> GE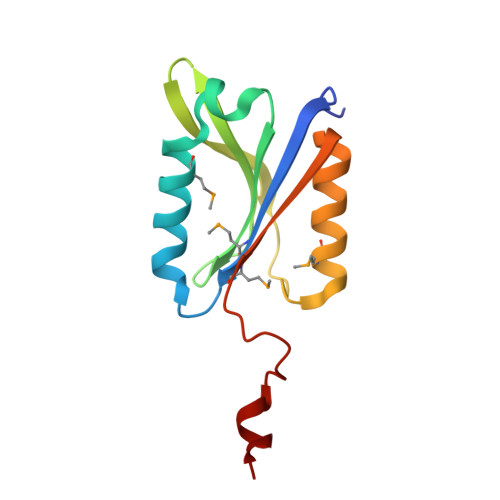TPEPRTTRTILVYMMANNSLNSFASKNIESMIEGATSKNLNGGNLIVYYAPAGSPPELLRIKEENGVVKKIHLKDYEKQNSADPDVMRSVIGEVVSQYPADSYGLVLWSHGTAWLPSDYQNKLK> MGQYKKLWYLLFAVLAVCFTILGYMGSEVYKKAPPYPEQVVSASGKVLMAKDDILAGQSAWQTTGGMEVGSVLGHGAYQAPDWTADWLHRELSAWLDLTAQQTYGKKFDEVSPEEQAVLKTRLADEYRNQSRIKEDGSVVISDTRVKAIESILPYYHGVYGDDPALQTTREHFAMKNNTLPSQEAREKLFDFFFWTSWSASTNRPDETFTYTNNWPHEPLINNVPTTENYMWSFTSVVLLLMGIGLLMWGYSFLTKHEEVEVPTEDPISKVQLTPSQKALGKYVFLTVALFVVQVLLGGLTAHYTVEGQGFYGIDEALGFEMSDWFPYALTRTWHIQSAIFWIATGFLTAGLFLAPIVNGGKDPKFQRAGVNFLYIALFIVVGGSYAGNFFALTHILPPEFNFWFGHQGYEYLDLGRFWQLLLMVGLLLWLFLMLRCTVSAFKEKGVDKNLLAIFVASMVGVGVFYAPGLFYGEKSPIAVMEYWRWWVVHLWVEGFFEVFATAAFAFVFYNMGFVRRSTATASTLAAAAIFMLGGVPGTLHHLYFSGSTSASMAIGACFSALEVVPLVLLGREAYEHWSYQHLSEWAKRLRWPLMCFVAVAFWNMIGAGVFGFLINPPISLFYIQGLNTSAVHAHAALFGVYGFLALGFVLLVARYLKPNVQFDDKLMTWGFWLLNGGLVGMIAISLLPVGVIQAYASITHGLWYARSEEFLQMEILDTLRWVRTAADLIFIGGAICVAIQATKIVFGRDK

A quinol-dependent nitric oxide reductase (qNOR) plays a critical role in the survival of the bacterium in the human host by combatting the host’s immune response. qNORs belong to the broader family of nitric oxide reductases (NORs). NORs are largely found as the essential component of anaerobic nitrate respiration, also known as denitrification, in the bacterial cytoplasmic membrane and catalyse the reduction of nitric oxide (NO) to nitrous oxide (N2O). Whilst cNORs are pre­dominantly found in denitrifying organisms as a respiratory enzyme, qNORs are also found in several pathogenic bacteria, including the Gram-negative, human-pathogenic bacterium N. meningitidis, as an enzyme that is responsible for the detoxification of NO produced by the host. High-resolution structure determination of N. meningitidis qNOR (NmqNOR) is of importance to provide a framework for developing a knowledge-based strategy for the design of new antibacterial agents, as well as to help to understand the chemistry of NO reduction, 2NO + 2 H+ + 2e− → N2O + H2O, at the heme and nonheme iron (FeB) binuclear centre.

The best, highly diffracting crystals of NmqNOR only grew in the presence of zinc sulfate, which was used in the crystallization condition. The crystals diffracted to ∼3 Å resolution, leading to a refined structure at 3.15 Å resolution in space group P212121, revealing only a monomer in the crystal lattice. Additionally, three Zn2+-binding sites were observed, of which the Zn1 and Zn2 binding locations were particularly important in order to understand the properties of the proton-transfer pathway. Zn1 is positioned near TMII, close to the predicted entry to the water channel, and is ligated by His257, Glu573, Glu576 and His577 [Fig. 2(b)]. The third binding site for Zn (Zn3) was observed near the periplasmic region where the zinc ion has three waters bound, in addition to His172, which itself is ligated to Glu709. The presence of zinc totally abolished the NO-reductase activity for both enzymes, while the presence of other divalent cations, such as magnesium and calcium, did not significantly reduce the activity. From the overall structure, TMII in the crystal structure moves significantly outwards compared with the cryo-EM structure. Alignment of the monomer and dimer structures of NmqNOR shows that Zn1 binding may cause the TMII loop region to splay away and into the symmetry-related molecule of the dimer, specifically clashing with TMX. The monomeric crystallographic structure of NmqNOR may result from disruption of the dimer interface owing to zinc binding near the dimer-stabilizing TMII region.> MKMASNDAAPSTDGAAGLVPESNNEVMALEPVAGAALAAPVTGQTNIIDPWIRANFVQAPNGEFTVSPRNAPGEVLLNLELGPELNPYLAHLARMYNGYAGGMEVQVMLAGNAFTAG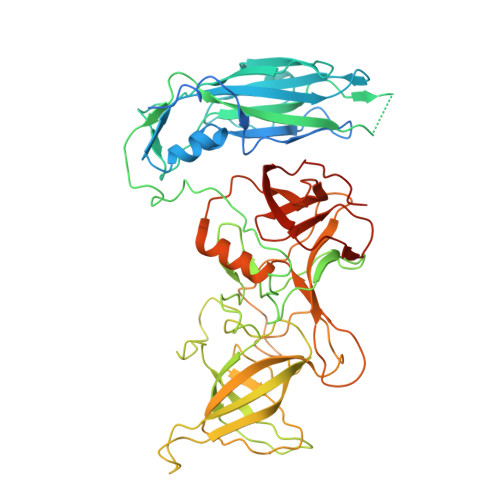KLVFAAVPPHFPVENLSPQQITMFPHVIIDVRTLEPVLLPLPDVRNNFFHYNQKDDPKMRIVAMLYTPLRSNGSGDDVFTVSCRVLTRPSPDFDFTYLVPPTVESKTKPFTLPILTLGELSNSRFPVSIDQMYTSPNEVISVQCQNGRCTLDGELQGTTQLQVSGICAFKGEVTAHLQDNDHLYNITITNLNGSPFDPSEDIPAPLGVPDFQGRVFGVITQRDKQNAAGQSQPANRGHDAVVPTYTAQYTPKLGQVQIGTWQTDDLKVNQPVKFTPVGLNDTEHFNQWVVPRYAGALNLNTNLAPSVAPVFPGERLLFFRSYLPLKGGYGNPAIDCLLPQEWVQHFYQEAAPSMSEVALVRYINPDTGRALFEAKLHRAGFMTVSSNTSAPVVVPANGYFRFDSWVNQFYSLAPMGTGNGRRRIQ Dextromethorphan | C18 H25 N O | 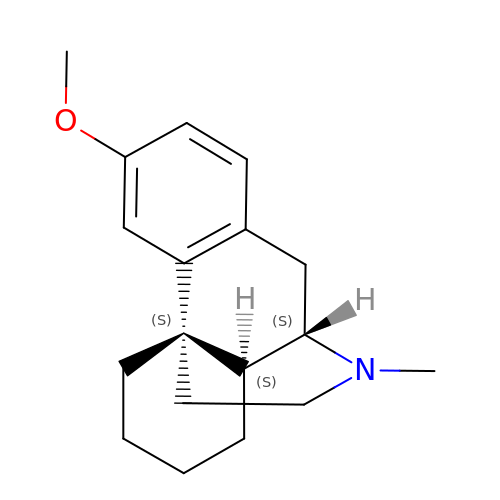MKXZASYAUGDDCJ-NJAFHUGGSA-N> MGSDKIHHHHHHMVKVLILGQGYVASTFVAGLEKLRKGEIEPYGVPLARELPIGFEDIKIVGSYDVDRAKIGKKLSEVVKQYWNDVDSLTSDPEIRKGVHLGSVRNLPIEAEGLEDSMTLKEAVDTLVKEWTELDPDVIVNTCTTEAFVPFGNKEDLLKAIENNDKERLTATQVYAYAAALYANKRGGAAFVNVIPTFIANDPAFVELAKENNLVVFGDDGATGATPFTADVLSHLAQRNRYVKDVAQFNIGGNMDFLALTDDGKNKSKEFTKSSIVKDILGYDAPHYIKPTGYLEPLGDKKFIAIHIEYVSFNGATDELMINGRINDSPALGGLLVDLVRLGKIALDRKEFGTVYPVNAFYMKNPGPAEEKNIPRIIAY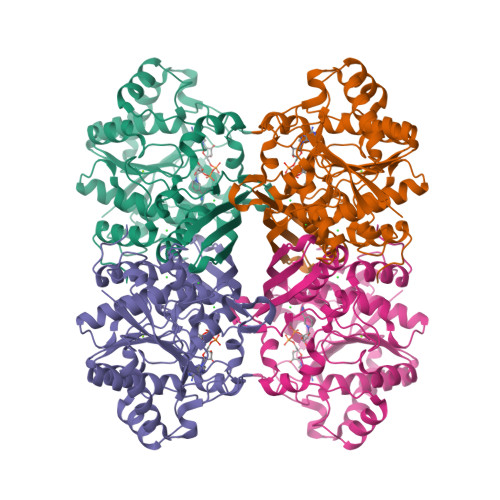EKMRIWAGLKPKWL>DPKLNFSWPVNVGPLNPHLYSPNQMFAQNMVYEPLVHYNADGTVGPWLAESWEASQDGRSYTFKLREDVKFSNGEVFDAAAVKANIDTVLQNRPRHNWLELVNQMVSAEVVGPYKVRINLKKPYYPLLQELSLPRPFRFIAPSQFKNGGTADGIVAPIGTGPWKLTETKLGEHDVFTRNDSYWGPKPAYEQITVKVIPDPNTRAIAFEAGEIDLIYGTEGP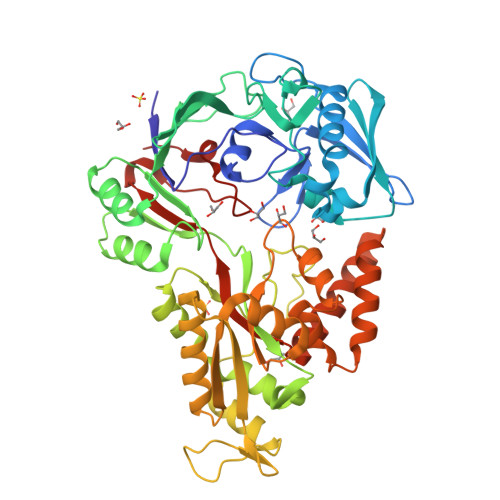ISPDTFERFQKMGIYNTELSEPLETRVLALNTNHGATKDLAVRKAINHAVDKDTMIATVLYGTQKRADTLFADNVPYANIGLKPYAFDPALAARLLDEAGWTAKASGDIREKDGQPLAIELCFIGTDAISKSMAEIVQADLRKVGIDVKLTGEEESSIYARQRDGRFDMIFNQTWGAPYDPHAFVSSMRVPSHADYQAQLGLPDKAKIDAEIGQVLVSTDETARQALYKDILTRLHEEAVYLPLTSVTAMAVAKPEVGKITFGAMSSEIPFEKLTPKAN[2x]>MGVPALFRWLSRKYPKIISPVIQDEDVDIDGESRPTRYEDPNPNGELDNLYLDMNGIVHPCSHPEHKPVPETEDEMMLDVFAYTENVIMMARPRKVIYIAVDGVAPRAKMNQQRSRRFRSAQDAKDANEKKAAELKEMEKKGEIIDDAIKNKKTWDSNAITPGTPFMHRLADSLRYWAAYKLTTDPGWSGIEVIISDASVPGEGEHKIMSYVRSLRSSPKHDPNTTHCIYGLAAALIFLGLATHEPHFKILREDVFAQDKKSYSLQDQLRMTDIERQELKDKKTPFLWLHLNILREYLQIELNVPGLSFPFDL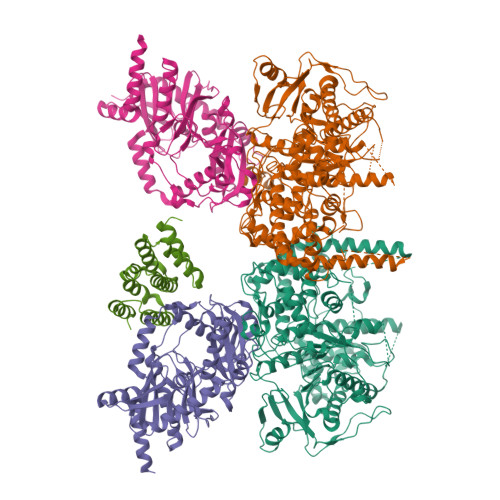EKSIDDWVFICFFCGNDFLPHLPSLDVRDNSITTLVTIWKQILPTMKGYLTTDGYLNLPAVERLLAELAKKEDYIFRKRYEDEKRSLENQKRRKLAQEQSSARSQNAPNISTGKDKAPLTPNQNIPLYTTSGESVGIKMTDSEMVNNSALITKANEANKSIAELLKQNLQNEINKKRKISNEEQEVVKESVEEVVEEEDDVLVTSDPEDSSTEILIPKNEEIRLWEPGYRKRYYETKFHTKDPQKVKKIARNMVQKYIEGVSWVLLYYYQGCPSWNWYYPYHYAPFAADFVNLSELKIEFVEGTPFRPYEQLMSVLPAASSHNLPDVFRSLMSDANSEIIDFYPEEFPLDMNGKKVIWQAIPLLPFIDENRLLKAVQSKYDQLTEDEKFRNTNRSEILVLGRSHSHYPTLVKELYEEGKDSYEFQVDSSGVSGVAIKLQSFDRSGVLRLPVKQLEGYRHYPDISNRDFLMVEFKQLPKSHAKSMILSGLIPHLRRLTQEDKDSILYGGTNFYGRNRFSPEENADFKQYIGPHGKSQYLPRQGGYKAFIQIHSDEAKGHRHGIYHGGSHTETEFRRGGGYHQHGNRGGRGGYQGNQGYQANSGGYQNSYQGSYQGGYRGGYQGGSQGRYQAGYQSGYQGGYQGEYKNGYQGGYQGNQGNQGYNRQTYNASKSGTLPMKRRHNSGPSSGLEVLFQ[2x];>GPGMSKEKILPLAARSKKAMLRQPKQVAYFSRDLNYKTHPDRSNLSYYYLPDGDIDNSIDLSVGSKHFLLGDSVELSKLDPILLALKEIEKESGAKTKDRIITWRGIMRKLLTLPYDSEEDFVLDVVSFDGQLFIQFNVPYLKSKDVQKQGDTEFHKKLQFSGYKFEKMATLPKPWPECTRKEIDSRAKSKCNNIEQYGAIVRTGISRIKILIGGAVACTADYYDENDPLSRYIELKTTRTINQYKDMIAFEKKLFRTWAQCFLLGIPKIIYGFRDDNCILRTVEEFSTNDIPLMVKNNPLNEQPKKENCYMSSINFYGAVVEWLNESVKDDQVWKLSYAKRNRQYLVLKEVTDENEKQQIVDSAIPAWFKEWRSELRNSEGNI[2x];> MSYSKDIVLEKLASLEETQISIQSIGQWCLFHHRHAPETVAIWSEFVGSTQTKKLAGLYLANEIIQQSRAKRKTTFLDEFAKVLPSTLEQIYPSMISTHQAKLKRIIDVWSQRKIFDSNLIHRLYQSIQDQKAYNGLSSSSSNSPPINSGDLAPEISSLSTLFNKISTLKSSTSLVVNQINEQYSSLFDSETLPGTDIYLKQLGDLSTLITSARSKSQETQELRESIINELKKLIQVQESWITKDAESSGSLDEKLATVQQKESELKEFINDVEEEDGVPQYAASSDEEGDENVSKKRKMESPPTETVDSGEQPTNPVHPQLSSILESLSRTTGLTPEPASTSDESATATQKQDETPVSSSINPALASLLSKLNGLEVLFQ>GITNSDFVIQQDNTKINNYQTNRPETSKRLFVSQAVEQQIAHIKQLLTNARLAWMFENCFPNTLDTTVHFDGKDDTFVYTGDIHAMWLRDSGAQVWPYVQLANKDAELKKMLAGVIKRQFKCINIDPYANAFNMNSEGGEWMSDLTDMKPELHERKWEIDSLCYPIRLAYHYWKTTGDASIFSDEWLTAIAKVLKTFKEQQRKEDPKGPYRFQRKTERALDTMTNDGWGNPVKPVGLIASAFRPSDDATTFQFLVPSNFFAVT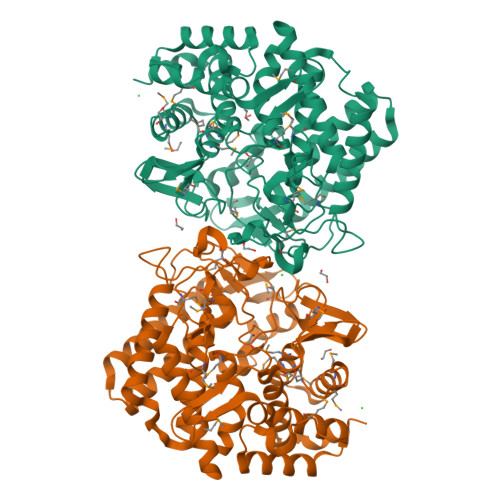SLRKAAEILNTVNKKPDLAKECTTLSNEVEAALKKYAVYNHPKYGKIYAFEVDGFGNQLLMDDANVPSLIALPYLGDVKVNDPIYQNTRKFVWSEDNPYFFKGTAGEGIGGPHIGYDMIWPMSIMMKAFTSQNDAEIKTCIKMLMDTDAGTGFMHESFHKNDPKNFTRSWFAWQNTLFGELILKLVNEGKVDLLNSIQ[2x]> MKILLIGMGGTIASVKGENGYEASLSVKEVLDIAGIKDCEDCDFLDLKNVDSTLI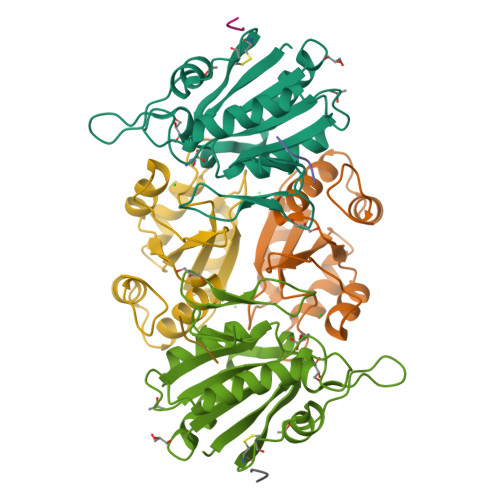QPEDWVDLAETLYKNVKKYDGIIVTHGTDTLAYTSSMISFMLRNPPIPIVFTGSMIPATEENSDAPLNLQTAIKFATSGIRGVYVAFNGKVMLGVRTSKVRTMSRDAFESINYPIIAELRGED;> MAVLVIKLIPGLSGDIFRAAVELGYRGIVIEGYGAGGIPYRGSDLLQTIEELSKEIPIVMTTQAMYDGVDLTRYKVGRLALRAGVIPAGDMTKEATVTKLMWILGHTNNVEEIKVLMRKNLVGELRD;>LVVN[2x]> VRPVADFSPSLWGDQFLSFSIKNQVAEKYAKEIEALKEQTRNMLLATGMKLADTLNLIDTIERLGISYHFEKEIDDILDQIYNQNSNCNDLCTSALQFRLLRQHGFNISPEIFSKFQDENGKFKESLASDVLGLLNLYEASHVRTHADDILEDALAFSTIHLESAAPHLKSPLREQVTHALEQCLHKGVPRVETRFFISSIYDKEQSKNNVLLRFAKLDFNLLQMLHKQELAQVSRWWKDLDFVTTLPYARDRVVECYFWALGVYFEPQYSQARVMLVKTISMISIVDDTFDAYGTVKELEAYTDAIQRWDINEIDRLPDYMKISYKAILDL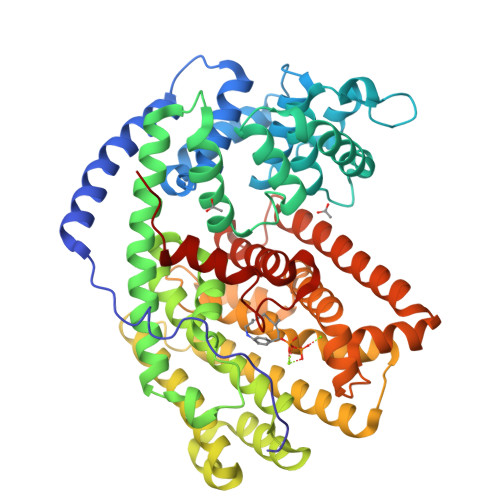YKDYEKELSSAGRSHIVCHAIERMKEVVRNYNVESTWFIEGYTPPVSEYLSNALATTTYYYLATTSYLGMKSATEQDFEWLSKNPKILEASVIICRVIDDTATYEVEKSRGQIATGIECCMRDYGISTKEAMAKFQNMAETAWKDINEGLLRPTPVSTEFLTPILNLARIVEVTYIHNLDGYTHPEKVLKPHIINLLVDSIKI>[4x]LGTENLYFQSNAYRALF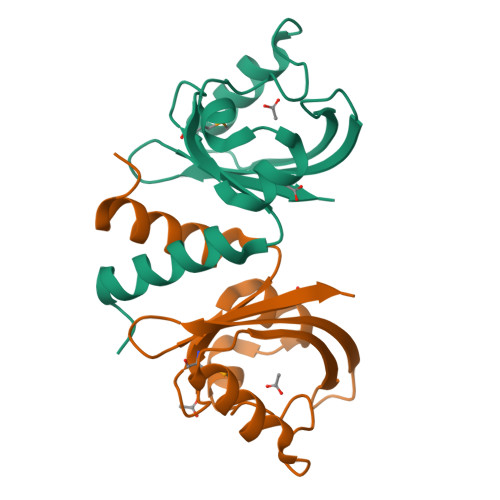EHAIDGIFIMDAEGHYLDVNPAICSAIGYTRDEFLALDWGVLSRGVDSGWAAASLARIVGGEPLREERTVWTRNGDQLTVELSAHLLPDGKILGIARDVS>[2x]MIKQRTLKNIIRATGVGLHSGEKVYLTLKPAPVDTGIVFSRTDLDPVVEIPARAENVGETTMSTTLVKGDVKVDTVEHLLSAMAGLGIDNAYVELSASEVPIMDGSAGPFVFLIQSAGLQEQEAAKKFIRIKREVSVEEGDKRAVFVPFDGFKVSFEIDFDHPVFRGRTQQASVDFSSTSFV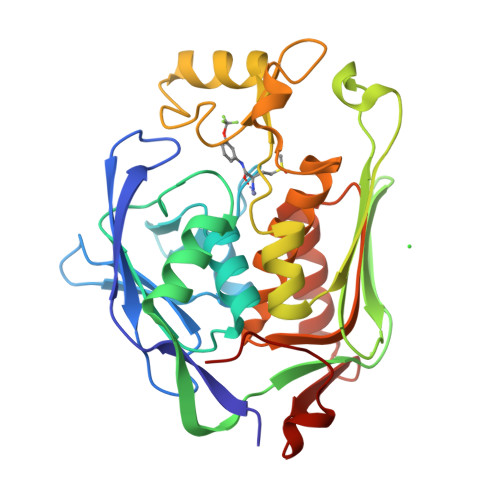KEVSRARTFGFMRDIEYLRSQNLALGGSVENAIVVDENRVLNEDGLRYEDEFVKHKILDAIGDLYLLGNSLIGEFRGFKSGHALNNQLLRTLIADKDAWEVVTFEDARTAPISYMRP> MTPIHILAFPFPAKGHINPLLHLCNRLASKGFKITLITTVSTLKSVKTSKANGIDIESIPDGIPQEQNHQIITVMEMNMELYFKQFKASAIENTTKLIQKLKTKNPLPKVLIYDSSMPWILEVAHEQGLLGASFFTQPCSVSAIYYHMLQGTIKLPLENSENGMVSLPYLPLLEIKDLPGVQQFEDNSEAVAELLADQFSNIDD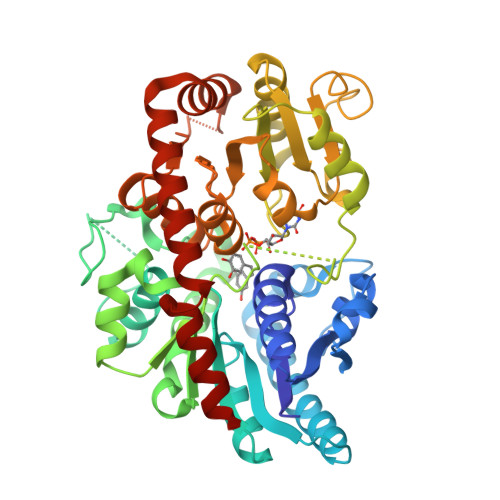VDYVLFNTFDALEIEVVNWMGSKWPILTVGPTAPTSMFFLDKKQKNYEDGRSINYLFETNTEVCMKWLDQREIDTVIYVSFGSLASLTEEQMEQVSQALIRSNCYFLWVVREEEENKLPKDFKETTSKKKGLVINWCPQLDVLAHKSVACFMTHCGWNSTLEALCSGVPMICMPQWADQTTNAKLIEHVWKIGVGVNKSDENGIVKREEIEDCIRQVIESERGKELKRNAIKWKELAKEAVSEGGSSCNNIQEFSSSLLFN>MGSSHHHHHHADESWRAPALVQELAAKGVEEPPSRYLLREQDRPDVKLVAAELPEPIPVVDLGRLDGAEEATKLRVALQNWGFFLLTNHGIEASLMDDVMNLSREFFNQPIERKQKFSNLIDGKHFQIEGYGTDRVVTQDQVLDWSDRLHLRVEPKEEQDLAFWPDHPESFRDVLHKYASGCKRIRDDIIQAMAKLLELDEDYFLDRFNEAPTFARFNYYPPCPRPDLVFGIRPHSDGGLLTILLVDKDVSGLQVQRDGKWSNVPATPHTLLINLGDTMEVMCNGIFKSPVHRVVTNAEKERISLAMLYSVNDEKDIEPAAGL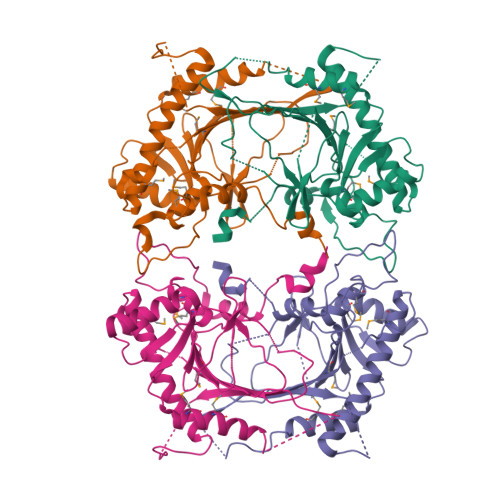LDENRPARYRKVSVEEFRAGIFGKFSRGERYIDSLRI[4x]>[4x]UGAGCX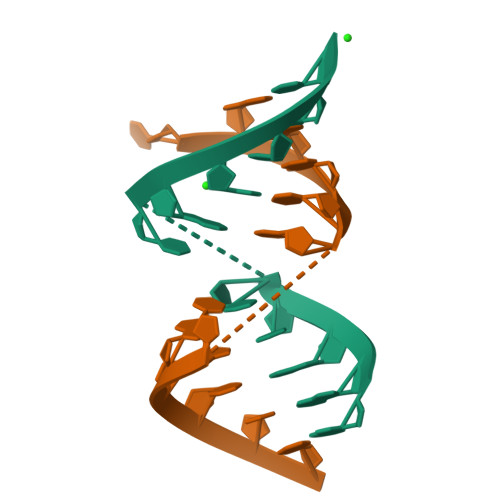CGGCUC> HHHHHHRSFFDFLKYKTIKEDDLNDVIEELRFQLLDSDVSYEVTEKILEDLKNNLIGKKVSRREEVEEIVINTLKKSITEILTKNQKTDLIEKIRSSGKKPFVIIFFGVNGVGKTTTIAKVVNMLKKNNLSTIIAASDTFRAAAQEQLAYHASKLEVQLIRGKYGADPASVAF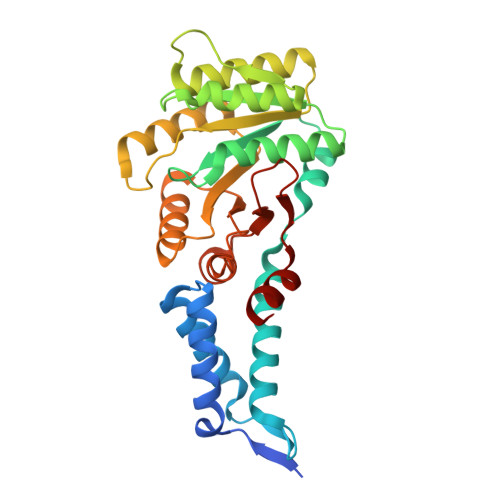DAISFAKSRNIDVVLIDTAGRMHIDSDLVEELKKVLRIAKPDFRILILDSLAGSDALEQARHFENNVGYDAVILTKVDADAKGGIALSLAYELKKPVVYMGVGQNYDDLIPFSPDWFVERIFS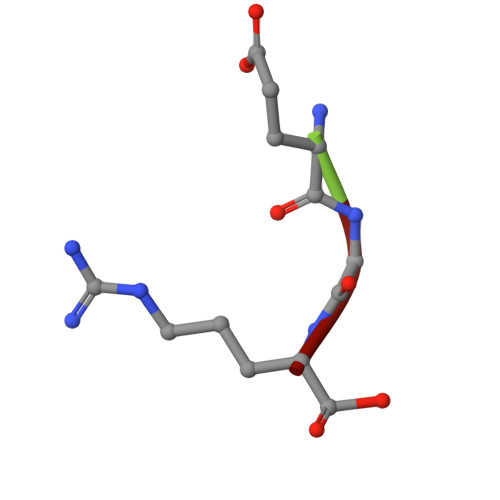> EGR>[2x]MGSSHHHHHHSSGLVPGRGSMKLTIERAALLKALGHVQSVVERRNTIPILSNILLSAEGDRLSFSATDLD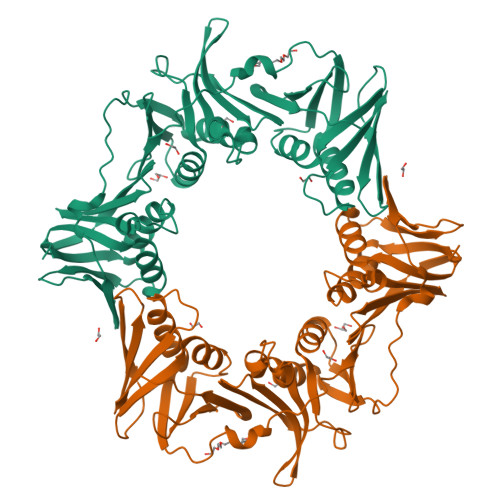MEIIDEGFAQIDVPGQITAPAHTLYEIVRKLPDGADVSLSFSGDDPRLVIQAGRSRFNLPVLPAGDFPVMSSDGLSSRIAVDTNELIRLIDKTRFAISTEETRYYLNGLYVHTVNEGGETKLRAVATDGHRLALAEMPAPEGAVGIPGVIVPRKTIAEARRLMESAGETVDLQVSPQKVRFEFGAAALTSKVIDGAFPDYMRVIPRDNAKILTLDNDLFAKAVDRVATISAEKSRSVKLAVEPGRITLTVRNMEAGQAVEEVEVDYDGEPFEIGFNARYLLDVCGQIAGPQAEFRFADPASPTLVVDPVDPGVKYVLMPLRV> MGS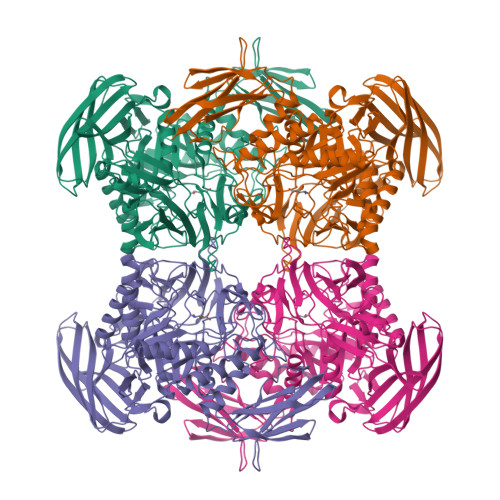SHHHHHHSSGLVPRGSMSLRQDILLNNNWNFRFSHQVQGDTRRVDLPHTWNAQDALAGKIDYKRGIGNYEKALYIRPEWKGKRLFLRFDGVNSIADVFINRKHIGEHRGGYGAFIFEITDLVKYGEKNSVLVRANNGEQLDIMPLVGDFNFYGGIYRDVHLLITDETCISPLDYASPGVYLVQEVVSPQEAKVCAKVNLSNRAADGTAELQVLVTDGTKVICKESRNVSLKQGADILEQLPLLIQKPRLWNGCEDPFMYQVSISLHKDGKQIDSVTQPLGLRYYHTDPDKGFFLNGKHLPLHGVCRHQDRAEVGNALRPQHHEEDVALMREMGVNAIRLAHYPQATYMYDLMDKHGIVTWAEIPFVGPGGYADKGFVDQASFRENGKQQLIELIRQHYNHPSICFWGLFNELKEVGDNPVEYVKELNALAKQEDPTRPTTSASNQDGNLNFITENIAWNRYDGWYGSTPKTLATFLDRTHKKHPELRIGISEYGAGASIYHQQDSLKQPSASGWWHPENWQTYYHMENWKIIAERPFVWGTFVWNMFDFGAAHRTEGDRPGINDKGLVTFDRKVRKDAFYFYKANWNKQEPMIYLAEKRCRLRYQPEQTFMAFTTAPEAELFVNGVSCGKQKADTYSTVVWKNVKLTSGENIIRVTTPGKKPLTDEVTVEYKEDREG> GPHMGGSMQKVSLRVTPRLVLEVNRHNAICVATNVPEFYNARGDLNIRDLRAHVKARMISSQFCGYVLVSLLDSEDQVDHLNIFPHVFSERMILYKPNNVNLMEMCALLSMIENAKSPSIGLCREVLGRLTLLHSKCNNLDSLFLYNGARTLLSTLVKYHDLEEGAATPGPWNEGLSLFKLHKELKRAPSEARDLMQSLFLTSGKMGCLARSPKDYCADLNKEEDANSGFTFNLFYQDSLLTKHFQCQTVLQTLRRKCLGSDTVSKIIP

BBRF2 is an EBV tegument protein that has putative homologues in all three herpesvirus subfamilies. Here, we report crystal structures of BBRF2 alone and in complex with BSRF1. BBRF2 binds EBV capsid protein MCP and capsid-associated protein BPLF1, whereas BSRF1 associates with EBV glycoproteins gB and gH/gL. These data elucidate the molecular basis of the functional association between BBRF2 and BSRF1, suggesting a role of BBRF2-BSRF1 in tethering EBV nucleocapsids to the Golgi membrane during secondary envelopment.

As crystallization of full-length BBRF2 was not successful, we modified the construct and determined the structure of an N- terminally truncated version with deletion of residues 1−16 (BBRF2Δ) at 1.6 Å. The phases were obtained by single anomalous diffraction using selenomethionine (SeMet) derivative, and the final model was refined to an Rfree of 0.189. ΒΒRF2Δ is monomeric both in solution and in the asymmetric unit of the crystal. BBRF2 has a compact globular architecture that represents a novel fold different from other known protein structures. Arg27 on the bulged loop between β1 and β2 forms salt bridges with Asp85 and Glu122, two highly conserved residues within herpesviruses. Glu122 further stabilizes the conformation of the bulged loop through two hydrogen bonds with the main chain nitrogen atoms of Leu28 and Val29, and Asp85 forms a salt bridge with His253 from η1. In addition, these residues and two deeply buried water molecules establish a comprehensive hydrogen bonding network with Asn123 and ambient main chain atoms. All of these interactions contribute to a prominent hydrophilic core at the center of BBRF2. According to the Dali server, the fold of BBRF2 does not resemble that of any existing protein structure. Thus, BBRF2 represents a novel protein domain, and we named it herpesvirus tegument fold 1 (HTF1).>[2x]GSHMVGETQRRFVLKQLDGQTAMPNVPYTITMANGEVIEGVTDAEGATQLLQKDAMNIAKVDMKHTKSPASAVAGIAAAVGAAVAVGKLLGGPDAEAGRALSEGEISLAKGVFGDSIDYSTVRLRDEDYVPWQGKDYVMAPNGHIYFGEELRGVADWSLESLQRQGLFIHEMTHVWQHQHGVNVLLVGAYQQARQFLLGDQYAYRLEPGKTLKDYNIEQQGDIVRDYFLAANAFGEASANSRFAGVLKNF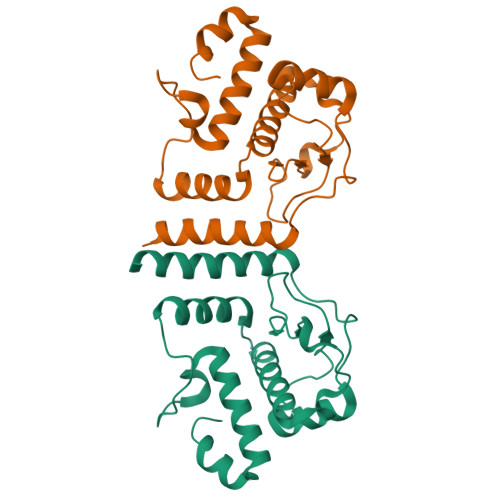PTGY The KSHV latency-associated nuclear antigen (kLANA) and the MHV68 mLANA (orf73) protein are required for latent viral replication and persistence. We solved the X-ray crystal structure of the C-terminal DNA binding domains (CTD) of kLANA and MHV-68 mLANA. The C-terminal domain (CTD) of LANA forms dimers, which bind two adjacent DNA sequences, the LANA binding sites (LBS1 & LBS2) in a single TR. Importantly, kLANA and mLANA CTD dimers undergo higher order oligomerization.

We also solved the crystal structure of a C-terminal fragment of MHV-68 LANA, mLANA(124–260), at a resolution of 2.14 Å, where a detailed structure was obtained for residues 130–260. It also is a native dimer, and the fold is very well conserved with kLANA. However, the structured CTDs of kLANA and mLANA share 28% sequence identity and the root-mean square deviation (r.m.s.d.) of the peptide backbone is only 2.2 Å. Between the two LANAs, the regions of highest structural conservation contain the entire β-barrel and the helices α2 and α3. Also mLANA CTD was observed to self-associate laterally where the dimers were arranged as linear chains. In kLANA, the interface is mostly hydrophobic, whereas it has a more hydrophilic character in mLANA. The angles between two neighboring LANA dimers range from 0° for mLANA, 72° for the kLANA pentameric rings to 90° for the kLANA tetrameric ring. Opposite to the DNA binding site, both kLANA and mLANA CTD contain a characteristic lysine-rich positively charged surface patch, which appears to be a unique feature of γ2-herpesviral LANA proteins. We have previously shown that residues 228–231 (KKLK), which are located on the basic surface of mLANA, influence the interactions with BRD2 and BRD4, and affect mLANA-mediated transcriptional activation. Likewise, the mLANA 4A mutant was incapable of establishing latency in the spleens of infected mice.

>[4x]GSKRYSRYQKPHNPSDPLPKKYQGMRRHLQVTAPRLFDPEGHPPTHFKSAVMFSSTHPYTLNKLHKCIQSKHVLSTPVSCLPLVPGTTQQCVTYYLLSFVEDKKQAKKLKRVVLAYCEKYHSSVEGTIVKAKPYFPLPE> SSSASVKGDVIYQIIIDRFYDGDTTNNNPAKSYGLYDPTKSKWKMYWGGDLEGVRQKLPYLKQLGVTTIWLSPVLDNLDTLAGTDNTGYHGYWTRDFKQIEEHFGNWTTFDTLVNDAHQNGIKVIVDFVPNHSTPFKANDSTFAEGGALYNNGTYMGNYFDDAT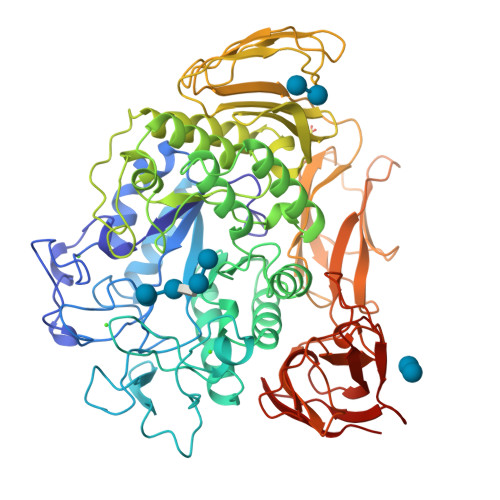KGYFHHNGDISNWDDRYEAQWKNFTDPAGFSLADLSQENGTIAQYLTDAAVQLVAHGADGLRIDAVKHFNSGFSKSLADKLYQKKDIFLVGEWYGDDPGTANHLEKVRYANNSGVNVLDFDLNTVIRNVFGTFTQTMYDLNNMVNQTGNEYKYKENLITFIDNHDMSRFLSVNSNKANLHQALAFILTSRGTPSIYYGTEQYMAGGNDPYNRGMMPAFDTTTTAFKEVSTLAGLRRNNAAIQYGTTTQRWINNDVYIYERKFFNDVVLVAINRNTQSSYSISGLQTALPNGSYADYLSGLLGGNGISVSNGSVASFTLAPGAVSVWQYSTSASAPQIGSVAPNMGIPGNVVTIDGKGFGTTQGTVTFGGVTATVKSWTSNRIEVYVPNMAAGLTDVKVTAGGVSSNLYSYNILSGTQTSVVFTVKSAPPTNLGDKIYLTGNIPELGNWSTDTSGAVNNAQGPLLAPNYPDWFYVFSVPAGKTIQFKFFIKRADGTIQWENGSNHVATTPTGATGNITVTWQN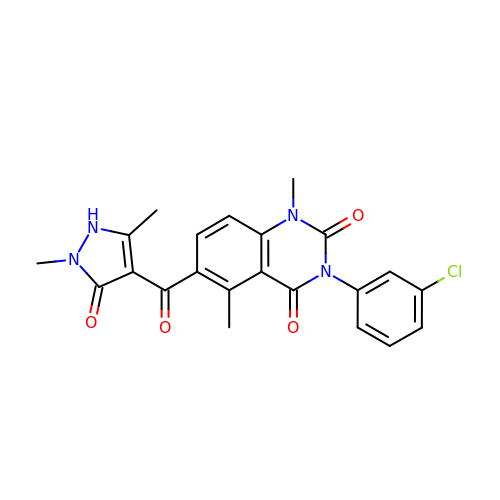3-(3-chlorophenyl)-6-[(2,5-dimethyl-3-oxidanylidene-1~{H}-pyrazol-4-yl)carbonyl]-1,5-dimethyl-quinazoline-2,4-dione | C22 H19 Cl N4 O4 | HYQZCGAYFSXSBE-UHFFFAOYSA-N> SNATTSSSDSEVIENVPVKVYY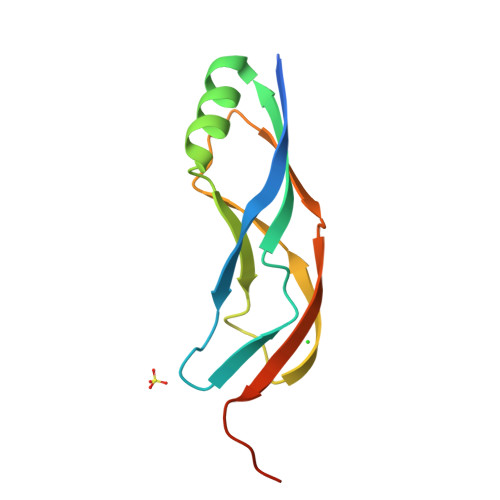DKTNLYISGIPETVTVTLSGPRSIVQSAKAQQDFTVYADLKNASIGTQEVKLQVKDVSDRLKVKVNPATVNVNVQEKVTKKFSVDVE> SMSTNGDDHQVKDSLEQLRCHFTWELSIDDDEMPDLENRVLDQIEFLDTKYSVGIHNLLAYVKHLKGQNEEALKSLKEAENLMQEEHDNQANVRSLVTWGNFAWMYYHMGRLAEAQTYLDKVENICKKLSNPFRYRMECPEIDCEEGWALLKCGGKNYERAKACFEKVLEVDPENPESSAGYAISAYRLDGFKLATKNHKPFSLLPLRQAVRLNPDNGYIKVLLALKLQDEGQEAEGEKYIEEALANMSSQTYVFRYAAKFYRRKGSVDKALELLKKALQETPTSVLLHHQIGLCYKAQMIQIKEATKGQPRGQNREKLDKMIRSAIFHFESAVEKKPTFEVAHLDLARMYIEAGNHRKAEENFQKL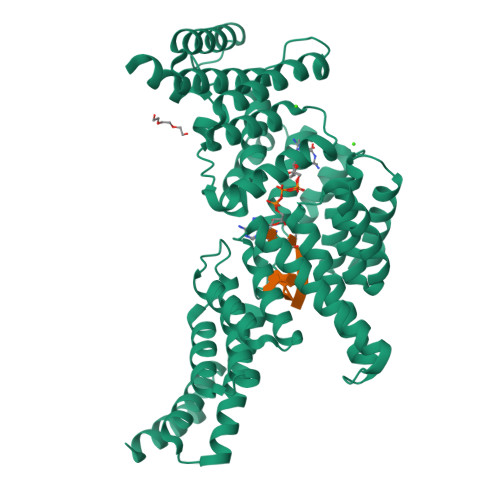LCMKPVVEETMQDIHFHYGRFQEFQKKSDVNAIIHYLKAIKIEQASLTRDKSINSLKKLVLRKLRRKALDLESLSLLGFVYKLEGNMNEAEEYYERAERLAADFENSVRQGP>MSCFVAKDGTQIYFKDWGSGKPVLFSHGWLLDADMWEYQMEYLSSRGYRTIAFDRRGFGRSDQPWTGNDYDTFADDIAQLIEH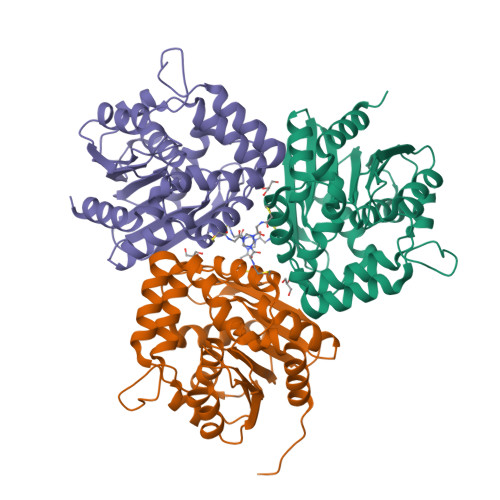LDLKEVTLVGFSMGGGDVARYIARHGSARVAGLVLLGAVTPLFGQKPDYPQGVPLDVFARFKTELLKDRAQFISDFNAPFYGINKGQVVSCGVQTQTLQIALLASLKATVDCVTAFAETDFRPDMAKIDVPTLVIHGDGDQIVPFETTGKVAAELIKGAELKVYKDAPHGFAVTHAQQLNEDLLAFLKRGSHHHHHH[15x]> QLLQPLPAEIKGTKLLAHWASGATITCIPESFLEDEQPIKKTLIKTIHGEKQQNVYYVTFKVKGRKVEAEVIASPYEYILLSPTDVPWLTQQPLQLTILVPLQEYQEKILSKTALPEDQKQQLKTLFVKYDNLWQHWENQVGHRKIRPHNIATGDYPPRPQKQYPINPKAKPSIQIVIDDLLKQGVLTPQNSTMNTPVYPVPKPDGRWRMVLDYREVNKTIPLTAAQNQHSAGILATIVRQKYKTTLDLANGFWAHPITPESYWLTAFTWQGKQYCWTRLPQGFLNSPALFTADVVDLLKEIPNVQVYVDDIYLSHDDPKEHVQQLEKVFQILLQAGYVVSLKKSEIGQKTVEFLGFNITKEGRGLTDTFKTKLLNITPPKDLKQLQSILGLLNFARNFIPNFAELVQPLYNLIASAKGKYIEWSEENTKQLNMVIEALNTASNLEERLPEQRLVIKVNTSPSAGYVRYYNETGKKPIMYLNYVFSKAELKFSMLEKLLTTMHKALIKAMDLAMGQEILVYSPIVSMTKIQKTPLPERKALPIRWITWMTYLEDPRIQFHYDKTLPELKHIPDVYTSSQSPVKHPSQYEGVFYTDGSAIKSPDPTKSNNAGMGIVHATYKPEYQVLNQWSIPLGNHTAQMAEIAAVEFACKKALKIPGPVLVITDSFYVAESANKELPYWKSNGFVNNKKKPLKHISKWKSIAECLSMKPDITIQHEKGHQPTNTSIHTEGNALADKLATQGSYVVN

A cleavage between the N-terminus of integrase (IN) and the C-terminus of the RNase H domain of RT produces mature IN and PR-RT from the Pol polyprotein. The mature PR-RT has all of the enzymatic functions of PR and RT [reviewed in [15]]. The PR-RTs of FVs are monomeric in solution and the RT component is responsible for converting the (+) FV ssRNA genome into dsDNA for integration into the host chromosome. The arrangement of the subdomains of PFV RT is similar to that of the p51 subunit of HIV-1 RT while the PR structurally resembles a single subunit of the catalytically active HIV-1 PR dimer.

In an effort to further investigate the structure and maturation of retroviral Gag-Pol and Pol polyproteins, we have determined and report here the crystal structure of the wild-type full-length PFV PR-RT protein at 2.9 Å resolution. The PR-RT we crystallized has a mutation in the active site of PR. The same crystallization condition that yielded the crystals of the CSH mutant did not produce usable crystals of the WT protein; relatively fragile, but usable, crystals of WT protein could be produced by modifying the crystallization conditions. Both the CSH mutant and WT PFV PR-RT crystallize as monomers with one copy in the asymmetric unit in space group C2. Despite differences in the unit-cell parameters, particularly along the x-axis, the structures of CSH and WT PR-RTs are highly superimposable (RMSD = 0.785 Å). Unless specifically indicated, the results we discuss here are from the WT protein structure. The connection subdomain is further tilted slightly towards the polymerase active site such that it sits almost parallel to the palm of the RT compared to its position in the p66 subunit of HIV-1 RT where the two subdomains are orthogonal. This compact fold allows helix L (K in HIV-1 RT) to pack against H, while helix O (L in HIV-1 RT) tilts towards the active site loop positioning T552 of PFV RT to form a hydrogen bond with Y314, and T556 with H236, while H507 forms a bifurcated hydrogen bond with S237 and N364. In the WT PFV PR-RT structure, there is a calcium ion from the crystallization buffer (which contains 100 mM Ca2+) that is chelated by the side chains of residues D601, E648, and D671, which define the RNase H active site. These residues are positional equivalents of D443, E478, and D498 of HIV-1 RNase H. In the PFV PR-RT structure, the RNase H domain occupies the opposite side of the DNA-binding cleft, with the active site pointing away from the putative nucleic acid-binding cleft.> MTTPVVANYENASMAADYIKRVSNVLPDIGIICGSGLGKLIEEIEERKVIPYINIPNFPKTTVAGHVGNLVLGSVGGRKIVAMQGRLHMYEGYSNQEIALPIRVMKLLGVRVLLITNLAGGINRKLKSGDFVLIKGHINFPGLGLNNVLVGPNQDEFGPRFPDLSNAYDRLLQQLALKIAQENDFQDLVHEGVYAFNGGPTYESPDESNMLLKLGCDVVGMSTVPEVIIACHCGIKVLAVSLIANNSILDAENDVSINHEKVLAVAEKRADLLQMWFKEIITRLPLD

Purine nucleoside phosphorylase (PNP) (E.C 2.4.2.1) is an enzyme responsible for reversible phosphorolysis of purine nucleosides, generating ribose-1-phosphate and their corresponding bases. Here, we characterize a newly identified isoform of S. mansoni PNP (SmPNP2) employing a combination of methodologies: ligand discovery by thermofluorescence, kinetic assays, high-performance liquid chromatography (HPLC) and X-ray crystallography. The crystal structure reveals this property appears to be related to the substitutions in the active site that induce the locking of the gate loop.

Soaking experiments using high ligand concentration was employed, resulting in four new SmPNP2 complexes with adenine, hypoxanthine, tubercidin, and cytidine. Using a soaking approach, three complexes were obtained: SmPNP2–tubercidin (7-deaza-adenosine), SmPNP2–hypoxanthine and SmPNP2–adenine (The composite omit maps of these ligands can be seen in S6 and S7 Figs, respectively). A totally different scenario is observed for the binding of adenine or hypoxanthine in the SmPNP2, where the bound base displays a 180° rotation in the Y axes followed a small rotation in the Z axes resulting in different interactions within Base Binding Site (BBS) in comparison to PNP1. The binding of adenine is similar to the hypoxanthine, however, a clear double conformation is observed for Glu203 (one of them is the canonical one), in this configuration the side chain of Glu203 interacts only with N7 (canonical conformation). The main reason for that is the steric constraints related to the presence of ribose group, which would argue against a similar conformation seen for adenine and hypoxanthine. This would mean that only after the glycoside bond cleavage the base could be free to rotate in the BBS and assume a non-canonical orientation.> MGGSHHHHHHGMASSVPIPGIKDISKLKFFYGFKYLWNPTVYNKIFDKLDLTKTYKHPEELKVLDLYPGVGIQSAIFYNKYCPRQYSLLEKRSSLYKFLNAKFEGSPLQILKRDPYDWSTYSNLIDEERIFVPEVQSSDHINDKF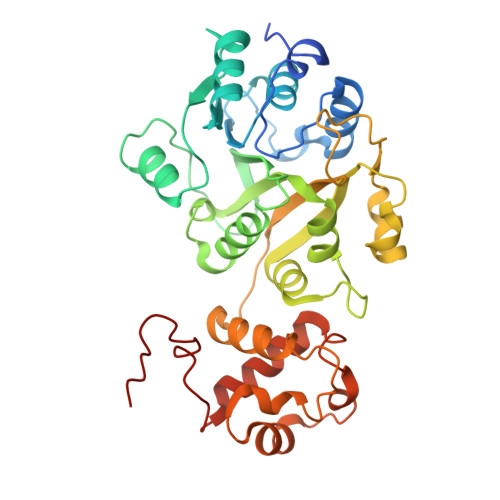LTVANVTGEGSEGLIMQWLSCIGNKNWLYRFGKVKMLLWMPSTTARKLLARPGMHSRSKCSVVREAFTDTKLIAISDANELKGFDSQCIEEWDPILFSAAEIWPTKGKPIALVEMDPIDFDFDVDNWDYVTRHLMILKRTPLNTVMDSLGHGGQQYFNSRITDKDLLKKCPIDLTNDEFIYLTKLFMEWPFKPDILMDFVDMYQTEHSG> MFSAGHKIKGTVVLMPKNELEVNPDGSAVDNLNAFLGRSVSLQLISATKADAHGKGKVGKDTFLEGINTSLPTLGAGESAFNIHFEWDGSM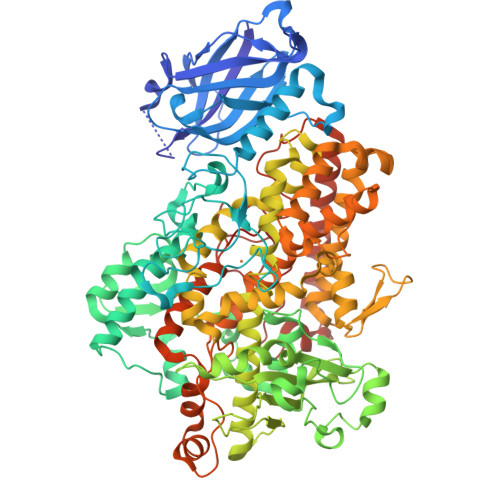GIPGAFYIKNYMQVEFFLKSLTLEAISNQGTIRFVCNSWVYNTKLYKSVRIFFANHTYVPSETPAPLVEYREEELKSLRGNGTGERKEYDRIYDYDVYNDLGNPDKSEKLARPVLGGSSTFPYPRRGRTGRGPTVTDPNTEKQGEVFYVPRDENLGHLKSKDALEIGTKSLSQIVQPAFESAFDLKSTPIEFHSFQDVHDLYEGGIKLPRDVISTIIPLPVIKELYRTDGQHILKFPQPHVVQVSQSAWMTDEEFAREMIAGVNPCVIRGLEEFPPKSNLDPAIYGDQSSKITADSLDLDGYTMDEALGSRRLFMLDYHDIFMPYVRQINQLNSAKTYATRTILFLREDGTLKPVAIELSLPHSAGDLSAAVSQVVLPAKEGVESTIWLLAKAYVIVNDSCYHQLMSHWLNTHAAMEPFVIATHRHLSVLHPIYKLLTPHYRNNMNINALARQSLINANGIAETTFLPSKYSVEMSSAVYKNWVFTDQALPADLIKRGVAIKDPSTPHGVRLLIEDYPYAADGLEIWAAIKTWVQEYVPLYYARDDDVKNDSELQHWWKEAVEKGHGDLKDKPWWPKLQTLEDLVEVCLIIIWIASALHAAVNFGQYPYGGLIMNRPTASRRLLPEKGTPEYEEMINNHEKAYLRTITSKLPTLISLSVIEILSTHASDEVYLGQRDNPHWTSDSKALQAFQKFGNKLKEIEEKLVRRNNDPSLQGNRLGPVQLPYTLLYPSSEEGLTFRGIPNSISI>ASEKEEILRKIKTQELAEAFNKVDRSLFLPENLKDYAYAHTHEALPILPGINTTALNLGIFMLDELDLHKGQKVLEIGTGIGYYTALIAEIVDKVVSVEINEKMYNYASKLLSYYNNIKLILGDGTLGYEEEKPYDRVVVWATAPTLLCKPYEQLKEGGIMILPIGVGRVQKLYKVIKKGNSPSLENLGEVMFGRIGGLYGFYDDYDDIEFRVNKLERQIK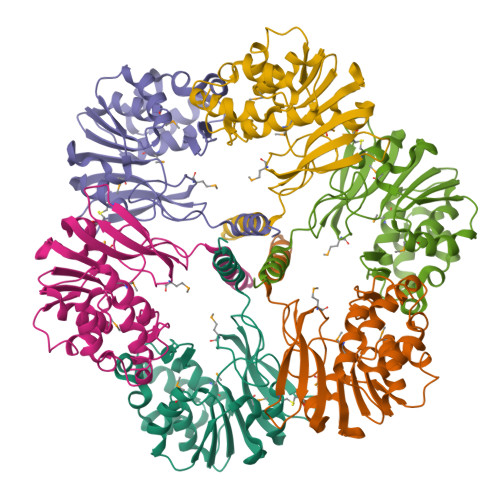SILDNLVKKT[4x]Here we describe a systematic approach to generating modular and rigid repeat protein oligomers with coincident C2 to C8 and superhelical symmetry axes that can be readily extended by repeat propagation. Repeat proteins are composed of an asymmetric structural motif that is concatenated several times in tandem within a single protein chain. From these building blocks, we demonstrate that a wide range of unbounded fibres can be systematically designed by introducing hydrophilic surface patches that force staggering of the monomers; the geometry of such fibres can be precisely tuned by varying the number of repeat units in the monomer and the placement of the hydrophilic patches. All multiplexes follow the naming convention CsHRN_Rr where s is the cyclic symmetry, HR stands for helical repeat, R is the number of repeats in a single chain and N is an index to differentiate between multiplexes of the same symmetry.

We determined the high-resolution structures of five designs from C2 to C6 symmetry by X-ray crystallography, cryogenic electron microscopy (cryoEM) or both. C4HR1_4r was solved at 3.3 Å by X-ray crystallography and ~3.7 Å by cryoEM; the two experimental structures are very close to the design model and to each other (r.m.s.d. values of 1.46 Å and 1.38 Å, respectively) with triangular-shaped repeat monomers with inner cavities lined by phenylalanines.

>[4x]MKKELYEFYFMPPLKQIEFLEELVNNPEKFKEFFKRLKEEPGAMELFLRNLYLMHPMVQIYFLELLVENPELFKLFFEYLEECPGAMEQFLLNLYLLHPMVQIEFLKLLVENPELFRLFFEYLKRCPGALELFKEIIELLDPIIQKYLKKLLEENPELKALVKEV>GSFVEMVDNLRGKSGQGYYVEMTVGSPPQTLNILVDTGSSNFAVGAAPHPFLHRYYQRQLSSTYRDLRKGVYVPYTQGKWEGELGTDLVSIPHGPNVTVRANIAAITESDKFFINGSNWEGILGLAYAEIARPDDSLEPFFDSLVKQTHVPNLFSLQLCGAGFPLNQSEVLASVGGSMIIGGIDHSLYTGSLWYTPIRREWYYEVIIVRVEINGQDLKMDCKEYNYDKSIVDSGTTNLRLPKKVFEAAVKSIKAASSTEK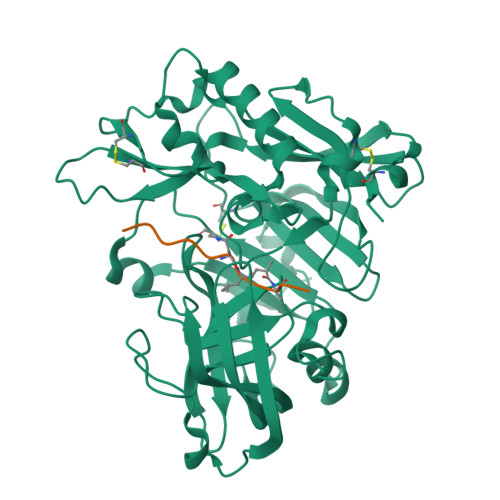FPDGFWLGEQLVCWQAGTTPWNIFPVISLYLMGEVTNQSFRITILPQQYLRPVEDVATSQDDCYKFAISQSSTGTVMGAVIMEGFYVVFDRARKRIGFAVSACHVHDEFRTAAVEGPFVTLDMEDCGYN[4x];>REWWSEVNXAEF[4x]> SNAGLIDESEQRLVDNIFEFEEKKIREIMVPRTDMVCIYESDSEEKILAILKEEGVTRYPVCRKNKDDILGFVHIRDLYNQKINENKIELEEILRDIIYISENLTIDKAL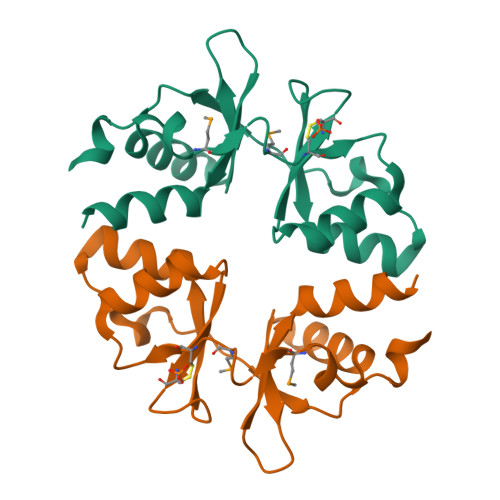ERIRKEKLQLAIVVDEYGGTSGVVTIEDILEEIVGEIQ> MGTSRDHMVLHEYVNAAGITGGSGGSENLYFQSMIHETILAIIIAFAISALLCPIIIPFLHKLKFGQQVRDDGPESHLKKQGTPTMGGLIILSSIIITSVFYIPSYPKIIPVL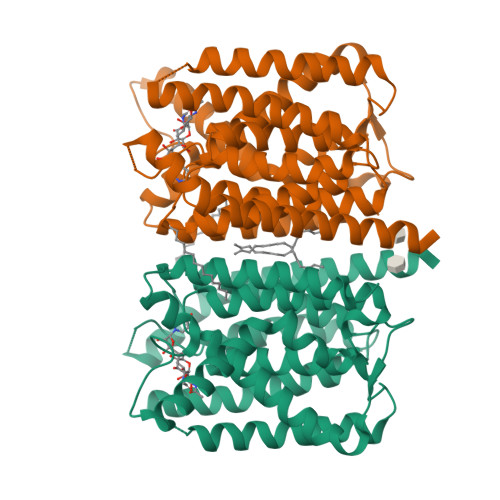FVTVGFGIIGFLDDYIKIVMKRSEGLKPMQKLVGQFIITGIFAWYLLNSGEVGTDMLIPFTGGFDGGSFLSLGIFFVPALFFIMLGTDNGVNFTDGLDGLCTSVTILVATFLTIVAIGEDMGISPITGAVVGSLLGFLLFNVYPAKVFMGDTGSLALGGFVAASCYMMRMPLFIPVIGLIYLVEVLSVIIQVTYFKRTGGKRIFKMAPIHHHFELCGWSETRVVAVFAIVTAILCMVAYLGLGSGSENLYFQSHHHHHHHHHH Colibactin, a DNA cross-linking agent produced by gut bacteria, is implicated in colorectal cancer. Its biosynthesis uses a prodrug resistance mechanism: a non-toxic precursor assembled in the cytoplasm is activated after export to the periplasm. Although the transmembrane domain is required for colibactin activation, its role in catalysis is unclear.

Crystal-packing interactions suggest that ClbP forms a dimer, and we confirmed this same dimeric species in solution using single-particle cryogenic electron microscopy (cryo-EM). To directly probe the oligomeric state of detergent-solubilized ClbP, we determined its structure by single-particle cryo-EM. The two-dimensional (2D) class averages derived from this analysis are consistent with the head-to-head dimer observed in the crystal lattice, and none suggests the presence of a monomeric species. After 2D and 3D classification, we selected 109,906 particles and generated a density map with a nominal resolution of 3.73 Å. The resulting dimeric ClbP structure is nearly identical to the crystallographic dimer (RMSD of 0.830 Å over 904 residues), except for a ~5° bend of each TMD toward the dimer axis. We also identified a branched density in the active site of both subunits that likely corresponds to co-purified phospholipids. Overall, our cryo-EM structure confirms that ClbP forms a stable dimer in solution through interactions matching those observed in the crystal lattice. In the dimer, the two periplasmic domains form a canopy over the cell membrane under which the active sites face each other. We discovered that ClbP forms a dimer that may promote the simultaneous activation of the two colibactin warheads, further supporting the proposed pseudodimeric structure of precolibactin.

>[2x]QEHEPIGAQDERLSTLIHQRMQEAKVPALSVSVTIKGVRQRFVYGVADVASQKANTLDTVYELGSMSKAFTGLVVQILIQEGRLRQGDDIITYLPEMRLNYQGKPASLTVADFLYHTSGLPFSTLARLENPMPGSAVAQQLRNENLLFAPGAKFSYASANYDVLGAVIENVTGKTFTEVIAERLTQPLGMSATVAVKGDEIIVNKASGYKLGFGKPVLFHAPLARNHVPAAYIHSTLPDMEIWIDAWLHRKALPATLREAMSNSWRGNSDVPLAADNRILYASGWFIDQNQGPYISHGGQNPNFSSCIALRPDQQIGIVALANMNSNLILQLCADIDNYLRIGKYADGAGDAITATDTLFVYLTLLLCFWGAVVVVRGAFRVYRATAHGPGKQQRLRLRVRDYIIALAVPGLVAAMLYVAPGILSPGLDWRFILVWGPSSVLAIPFGIILLAFVLTLNHQIKRILLHNKEWDDEHHHHHHHHHH N-[3-({4-[(3-aminopropyl)amino]butyl}amino)propyl]acetamide 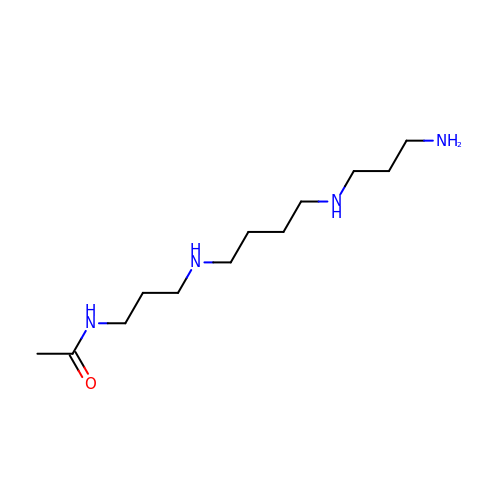| C12 H28 N4 O | GUNURVWAJRRUAV-UHFFFAOYSA-N> SMAEDTGVRVELAEEDHGRKSTIALRLWVEDPKKLKGKPKDNGAIEFTFDLEKETPDEVAQEMIESGF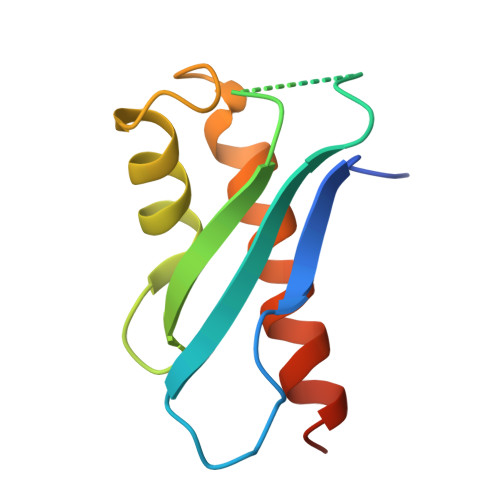FHESDVKIVAKSIRDRVALIQWRRERIWPA>SMTTNVGDSTLADLLDHSCTSGSGSGLPFLVQRTVARQITLLECVGKGRYGEVWRGSWQGENVAVKIFSSRDEKSWFRETELYNTVMLRHENILGFIASDMTSRHSSTQLWLITHYHEMGSLYDYLQLTTLDTVSCLRIVLSIASGLAHLHIEIFGTQGKPAIAHRDLKSKNILVKKNGQCCIADLGLAVMHSQSTNQLDVGNNPRVGTKRYMAPEVLDETIQVDCFDSYKRVDIWAFGLVLWEVARRMVSNGIVEDYKPPFYDVVPNDPSFEDMRKVVCVDQQRPNI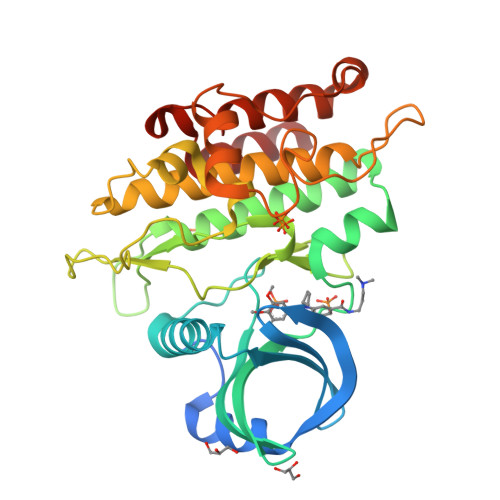PNRWFSDPTLTSLAKLMKECWYQNPSARLTALRIKKTLTKID[2x]>MKRFFNRFYLDTGIIADPSQRSLASRVSAFLVQGAVAFSLLGTIGVDTSPLIAAAGVTGATIVFACKDFGTNFVASIVLSGQQSIRTGNLVCIGTGLNVVKGKVVDWDTRYLYLRSSEGHLLHVPNNMVLNSVVTWEQEKKQNPHETDLPKQDVVKAPGDNAAKQS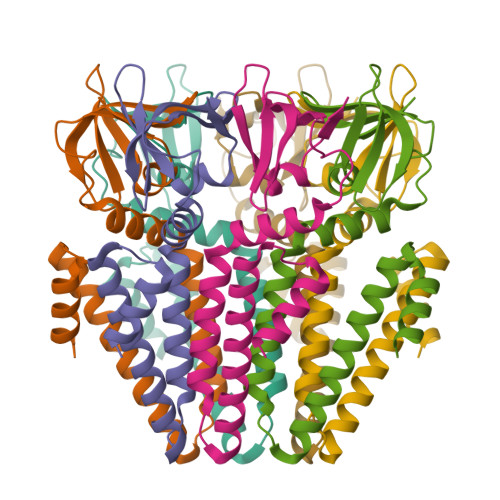NSLEVLFQ[7x]>MNSSLPSLRDVFANDFRIGAAVNPVTIEMQKQLLIDHVNSITAENHMKFEHLQPEEGKFTFQEADRIVDFACSHRMAVRGHTLVWHNQTPDWVFQDGQGHFVSRDVLLERMKCHISTVVRRYKGKIYCWDVINEAVADEGDELLRPSKWRQIIGDDFMEQAFLYAYEADPDALLFYNDYNECFPEKREKIFALVKSLRDKGIPIHGIGMQAHWSLTRPSLDEIRAAIERYASLGVVLHITELDVSMFEFHDRRTDLAAPTSEMIERQAERYGQIFALFKEYRDVIQSVTFW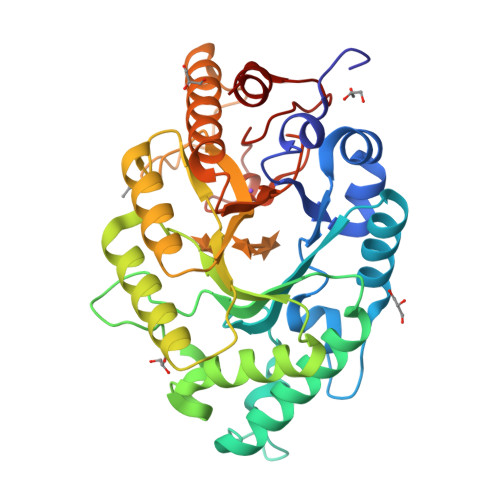GIADDHTWLDNFPVHGRKNWPLLFDEQHKPKPAFWRAVSV[2x]>[2x]MKFTVEREHLLKPLQQV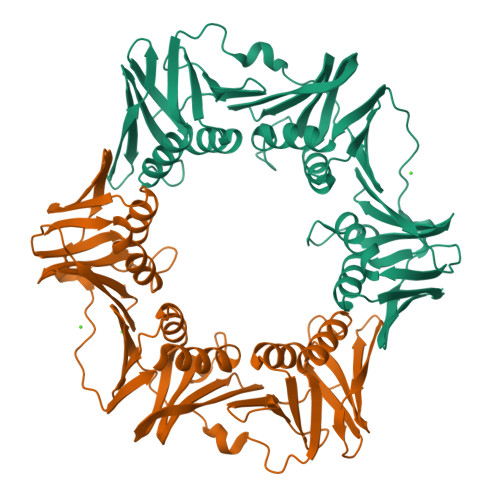SGPLGGRPTLPILGNLLLQVADGTLSLTGTDLEMEMVARVALVQPHEPGATTVPARKFFDICRGLPEGAEIAVQLEGERMLVRSGRSRFSLSTLPAADFPNLDDWQSEVEFTLPQATMKRLIEATQFSMAAAAAAYYLNGMLFETEGEELRTVATDGHRLAVCSMPIGQSLPSHSVIVPRKGVIELMRMLDGGDNPLRVQIGSNNIRAHVGDFIFTSKLVDGRFPDYRRVLPKNPDKHLEAGCDLLKQAFARAAILSNEKFRGVRLYVSENQLKITANNPEQEEAEEILDVTYSGAEMEIGFNVSYVLDVLNALKCENVRMMLTDSVSSVQIEDAASQSAAYVVMPMRL>MATEQIQHIAIVGCVHGKYREMYRQLSEYEKSTGKEISFVICTGDMQTLRYEADLVYLKVPPKYKQMGDFHLYYEGKEKAPYLTLFIGGNHESSNVLLHLYNGGFVCFNMYYLGVCSCININGLRIVGVSGIYKSFDEKKPYTYPPSPNDVVSLFHTRNYVIQMLSNLSQSSQIDISLSHDWPQGIVMKGNYKQLYRFQPGFKKDGASLGSPINKVILNTLKPKYWISGHMHCEYHAEEGPTHFIALGKIGYKNAISYLDLPLKQKTDLEYDKDWVCNLIMTWPAFSNKAQFPDLSYSISELLSKRTKELDKKIIELWEKYIGLKIIYDSDTFDIQFTSRRFYIEKIYNELNINHHHHHH[5x]

The spliceosome excises introns from nascent messenger RNA (1) in the form of a lariat containing an unusual 2′,5′-phosphodiester linkage (2). Hydrolysis of this linkage is rate-limiting in lariat degradation after splicing, and is required for efficient maturation of many small nucleolar RNAs (snoRNA) and micro RNAs (mirtrons) that are derived from intronic RNA. Dbr1 is tuned to hydrolyze 2′,5′-phosphodiester RNA linkages in branched RNA and not the considerably more abundant canonical 3′,5′-phosphodiester linkages, although the molecular basis for this selectivity has remained elusive for several decades despite extensive biochemical characterization of the enzyme. Sequence analyses predict Dbr1 consists of an N-terminal domain belonging to the metallophosphoesterase (MPE) superfamily of enzymes and a C-terminal domain (CTD) lacking detectible sequence similarity to any other class of protein.

To address this gap in knowledge, the 3D structure of the Dbr1 enzyme from the unicellular protist Entamoeba histolytica was determined using single crystal X-ray diffraction. Dbr1 crystallized in space group P212121 with five molecules in the asymmetric unit. The five protomers in the asymmetric unit are virtually identical, superimposing with an average root mean square deviation (RMSD) of 0.16 Å for backbone atoms. The observed packing interactions in the crystal are limited, consistent with analytical ultracentrifugation sedimentation velocity data indicating the protein exists as a ∼42 kDa monomer in solution. The N-terminal 261 residues adopt the MPE fold, characterized by adjacent α and β metal-binding pockets. However, the α pockets in the four Dbr1 structures determined in this work are devoid of metal ions and an invariant cysteine residue (Cys14) in Dbr1 enzymes replaces the aspartic acid present in virtually all other members of the MPE superfamily. The Mn2+ ion in the β pocket is coordinated in an octahedral geometry by the side chains of Asp45, Asn90, His180, His230, a water molecule and a sulfate ion coming from the crystallization liquor. As predicted in previous studies on the yeast enzyme, a conserved histidine residue (His91) is poised to protonate the leaving group 2′O during hydrolysis of the 2′,5′-phosphodiester linkage in lariat RNA. The electrostatic environment surrounding the active site is compatible with the binding of negatively charged RNA.>[2x]MRMTWNFHQ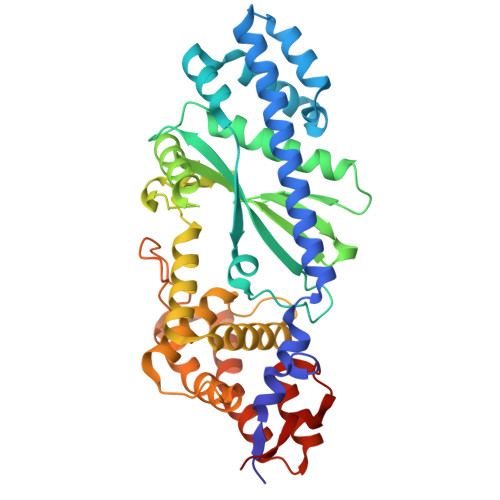YYTNRNDGLMGKLVLTDEEKNNLKALRKIIRLRTRDVFEEAKGIAKAVKKSALTFEIIQEKVSTTQIKHLSDSEQREVAKLIYEMDDDARDEFLGLTPRFWTQGSFQYDTLNRPFQPGQEMAIADGTYMPMPIFESEPKIGHSLLILLVDASLKSLVAENHGWKFEAKQTCGRIKIEAEKTHIDVPMYAIPKDEFQKKQIALEANRSFVKGAIFESYVADSITDDSETYELDSENVNLALREGDRKWINSDPKIVEDWFNDSCIRIGKHLRKVCRFMKAWRDAQWDVGGPSSISLMAATVNILDSVAHDASDLGETMKIIAKHLPSEFARGVESPDSTDEKPLFPPSYKHGPREMDIMSKLERLPEILSSAESADSKSEALKKINMAFGNRVTNSELIVLAKALPAFAQE>MGKDYQVLGKNKVKVDSLEKVMGTAKFAADYSFPDMLYAGVFRSTVPHARIVSLDLSKARAIDGVEAVLDYHAIPGKNRFGIIIKDEPCLVDDKVRRYGDAIAVVAAQTPDLVQEALDAITIEYEELEGIFTMERALEEDSPAIHGDTNIHQVKHLEYGDVDAAFKQCDIVVEDTYSTHRLTHMFIEPDAGVSYYDNEGMLTVVVSTQNPHYDRGEVAGMLALPNSKVRIIQATTGGGFGGKLDLSVQCHCALLTYHTKKPVKMVRSREESTTVSSKRHPMTMHCKTGATKDGRLQAVQVEMFGDTGAYASYGPAVITRATVHCMGPYVVPNVRVDAKFVYTNNPMSGAFRGFGVPQASVCHEGQMNALAKALGMDPIDIRILNAHQVGAKLATGQVLENSVGLIETLEKAREKAVEVMGYEKTR[2x];>[2x]MKKRGKGVGSMWYGIGNTGLPNPAAAFVEIHGDGSANVMFGAADIGQGSGTAMAQIAAEELGLDYEKIH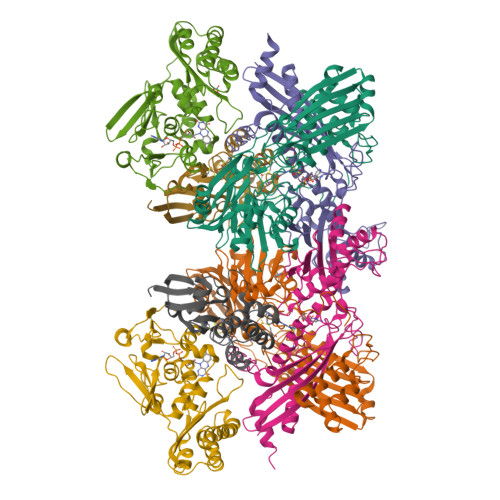VTWGDTMVTPDGGATSASRQTLITGNAVILACRQAKETLAKTAAEKLDCAPEELSFRDNTVFITADPERSMTYGELMAAMKAAGRMAVGAGSYNPNTTGLAPENMSGIPFEVYSYATTIAEVEVDTETGEVDVLKVVSAHDVGTPINRSMVEGQIEGGVTMGQGFVLMEEIEVNTKNGAIKNPSMSKYIIPSNRDVPEIHSILVESEGGPGPFGAKGVGEPALIPMIPAVVAAIEDALGTRFTHTPIMPKDIVAAVKAQEK;>[2x]MKDFEFFAPKTLEEAKGLLHQYKDVPPAIIAGGTDLVIEINDRWEKPDVVIDIKKLKELEYIRVEENTIHIGALSTFTQIENHPFIRSHVRALYKAASQVGSPQIRNLGTIGGNLSTSSVAGDGVSAMTTLDATVVLESVRGTRQMKLTDFFDGEGFKRRNALEADEIMTEVIIDRPDAHSASAFYKLAKRKSLAISVIGGGMAVKVDDAGVCTWASMRGGCIGRYPLHFKQAEEMLVGAPLTMETMEATLPILHDTVYDMARARPSVLYKKESVQGVFKKLFVDILDQLEGGCNE;>MNKITINLNLNGEARSIVTEPNKRLLDLLREDFGLTSVKEGCSEGECGACTVIFNGDPVTTCCMLAGQADESTIITLEGVAEDGKPSLLQQCFLEAGAVQCGYCTPGMILTAKALLDKNPDPTDEEITVAMSGNLCRCTGYIKIHAAVRYAVERCANAAA[2x]>GSMTSKIALFDQTLIASLLQPLSLNQPDFKAYKTKVKLKISEQRNETSGEKELKFEISRSDDFEFLFSETLNNEKYQILARDHDLTVDFDAFPKVIIQHLLCKNTEINIILDAEKNFCSFELFSGKIF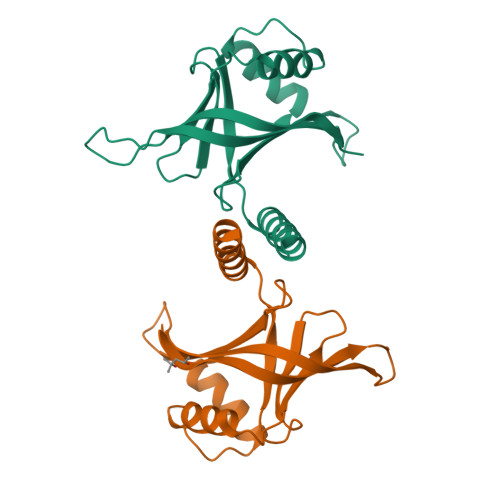SIKLHAVRGDHLISHLLKICSSQAVKLSTFYKSADELASLRQKCGDLEKQVEKLS[4x]>MIMDKSIPKATAKRLSLYYRIFKRFNTDGIEKASSKQIADALGIDSATVRRDFSYFGELGRRGFGYDVKKLMNFFAEILNDHSTTNVMLVGCGNIGRALLHYRFHDRNKMQISMAFDLDSNDLVGKTTEDGIPVYGISTINDHLIDSDIETAILTVPSTEAQEVADILVKAGIKGILSFS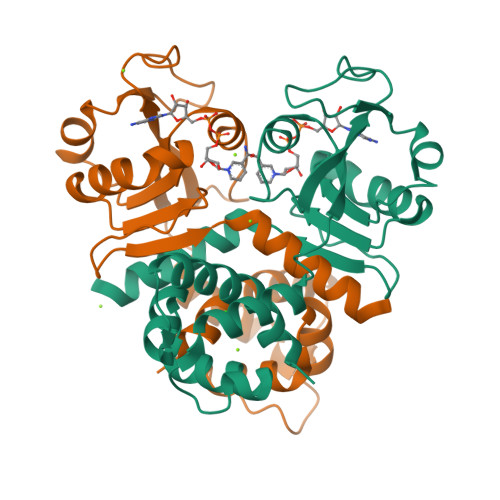PVHLTLPKDIIVQYVDLTSELQTLLYFMNQQR[2x]>WSHPQFEKENLYFQGMSRKFDFITKNNLWTNEQRDAADKVLAEIDSLGLEMIRLSWADQYGLLRGKSLTVASLKSAFKEGSEVAIGPFFFDLVSSMVFNLFTTAGDFEDELSGNPTVVMVPDPTTFKVLPWADKTGWMLADLHWKSGEPFPLCPRGIMKKAVKSLSDEGYLFKCGIELEWYLTKIVDRSLSPESLGAPGVQPDAIQVQPVAQGYSVLLEHHLDQVDDIMSKVRKGLLELNLPLRSIEDEWAPSQMETTFDVMEGLEAADAALLIKSAIKQICSRHGYHATFMCKPAINGFFASGWHMHQSLVDKDTRKNLFIPSEGEVLSPLGRAYAGGLLANGSAASSFTTPTVNGYRRRQPYSLAPDRRAWAKDNKAAMVRVVSATGDPASRIENRIGEPGANPYLYMASQIVSGLDGIKNKKDPGELQESPYDAQVPMLPTTLAEALDALEHDSELFRSCFGDTFIKYWLQLRRSEWARFLDAEGAEAAEPTGAVTQWEQKEYFNLL[6x]

A glutamine synthetase-like (GS-like) enzyme (NpaA1) initiates 1NA glutamylation, and this enzyme exhibits a broad substrate selectivity toward a variety of anilines and naphthylamine derivatives. During γ-glutamylation of 1NA, the 1NA consumption (0.16 mmol) was almost equivalent to the total accumulation of γ-glutamylated 1NA (0.157 mmol). In view of the above analyses, NpaA1 was established as a γ-glutamylnaphthylamide synthase catalyzing ligation of 1NA and L-glutamate to form γ-glutamylated 1NA. The crystal structure of apo-NpaA1 and two complexes with substrates or substrate analogs were obtained. The binding pocket is located at the interface between adjacent subunits, and the bifunnel channel similar to GS protein refers to a structural feature characterized by two distinct channels that converge into the common active site.

When the ATP analog AMPPNP binds to NpaA1, an additional Mg2+ binds to the active site, facilitating the binding of the AMPPNP phosphate group. The coordinating residues involved in ATP, glutamate, and Mn2+ binding are highly conserved between NpaA1 and GS.> SG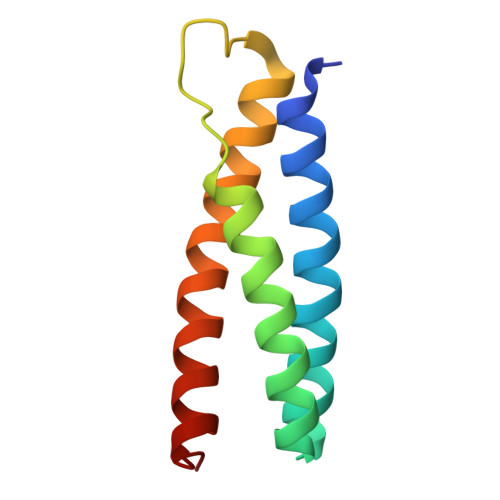EPAEIKIIREAYKKAFLFVNKGLNTDELGQKEEAKNYYKQGIGHLLRGISISSKESEHTGPGWESARQMQQKMKETLQNVRTRLEILEKGLAT3-[1-[[4-(piperidin-1-ylmethyl)phenyl]methyl]indol-6-yl]-1~{H}-pyrazol-5-amine | C24 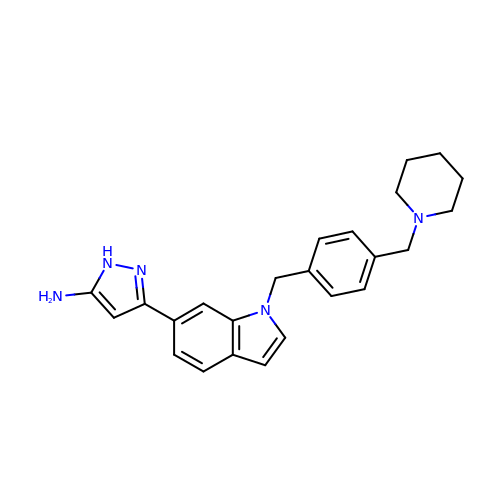H27 N5 | VDYQWEHGAZCAGH-UHFFFAOYSA-N> MSTVHEILCKLSLEGDHSTPPSAYGSVKPYTNFDAERDALNIETAVKTKGVDEVTIVNILTNRSNVQRQDIAFAYQRRTKKELPSALKSALSGHLETVILGLLKTPAQYDASELKASMKGLGTDEDSLIEIICSRTNQELQEINRVYKEMYKTDLEKDIISDTSGDFRKLMVALAKGRRAEDGSVIDYELIDQDARELYDAGVKRKGTDVPKWISIMTERSVCHLQKVFERYKSYSPYDMLESIKKEVKGDLENAFLNLVQC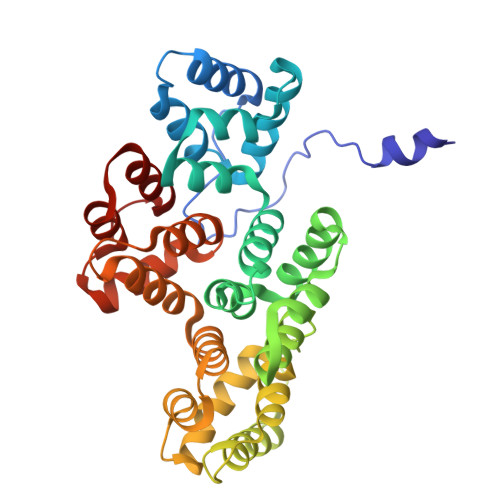IQNKPLYFADRLYDSMKGKGTRDKVLIRIMVSRSEVDMLKIRSEFKRKYGKSLYYYIQQDTKGDYQKALLYLCGGDD The present study focuses on the ancestor SMS from the hyperthermophilic archaeon Methanocaldococcus jannaschii. Biochemical and structural studies showed that SMS is made of a SmsC2B2 heterotetratmer wherein the SmsC subunit hosts both ATP and [Fe-S] cluster binding sites. With respect to the six components of the SUF system, SMS has only two components, SmsC and SmsB, encoded by the smsCB operon. The SmsC subunit, consisting of a RecA-like domain and a helical domain, contains all the structural motifs of the nucleotide-binding (NBD) subunits of the ABC ATPases (i.e., Walker A, Walker B, ABC signature, D-, Q-, and H-loops).

Incubation of SmsC with excess of adenosine-5′-[(β,γ)-methyleno]triphosphate (AMP-PCP) led to SmsC dimer formation. The SmsCK45R variant was not able to form homodimers upon AMP-PCP binding, consistent with the notion that binding of ATP is required for dimerization of SmsC. The interface between the SmsC subunits is weaker (the buried surface area is 730 Å2), and likely susceptible to changes upon ATP binding and hydrolysis. Such a conformational change is supported by the structure of the SmsC2 bound to an AMP-PN, which exhibits a “close” conformational state, similar to that observed in many structures of ABC transporters. The SmsC subunits rearrange again to transiently form a tight dimer as seen in the SmsC2 structure favoring ATP hydrolysis (intermediate 3), after which ADP and Pi leave SmsC and SmsC is reset to engage into assembling a new [Fe-S] cluster (intermediate 1).

>[2x]GEFMVSIMLLKVEDLHVYRGNREILKGVNLTVEENEIHAIIGPNGAGKSTLAYTIMGISGYKPTKGRIIFKGVDIIDKNITERARMGMTLAWQEPARFEGIKVKNYLMLGMNEKYKKDKEIAEEKIREALKLVNLDPDKYLDRYVDETLSGGERKRIELASIICMEPDLAILDEPDSGIDIVSFDEIKRVFDYLKDKGCSLLVITHREELAEHADRVSLICAGEVIKSGDPKEVGEFYKKECGKCYKKVPDGK> IIGGREVIPHSRPYMASLQRNGSHLCGGVLVHPKWVLTAAHCLAQRMAQLRLVLGLHTLDSPGLTFHIKAAIQHPRYKPVPALENDLALLQLDGKVKPSRTIRPLALPSKRQVVAAGTRCSMAGWGLTHQGGRLSRVLRELDLQVLDTRMCNNSRFWNGSLSPSMVCLAADSKDQAPCKGDSGGPLVCGKGRVLAGVL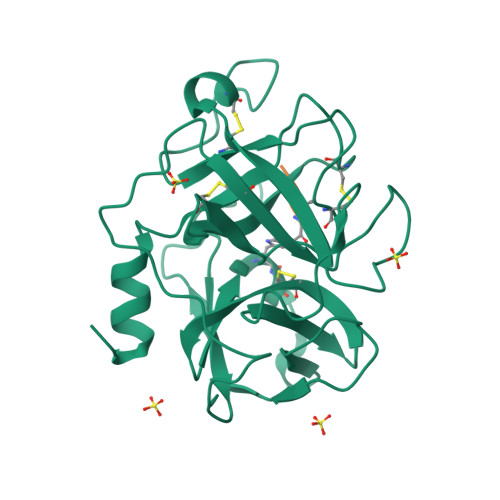SFSSRVCTDIFKPPVATAVAPYVSWIRKVTGRSALEHHHHHH>GSHMSMYNMDLDKVIRKINKKGARTVGLQFPEGLKMQAVKIAKAIESQTPATVIISGDPCFGACDVSDYKMKGSVDLIVHYGHTPLPLKYEVPTLFIEAFSNIDVKKDLEKCLEKLEDYSKIALVTTTQHLHLLNEIKDYLEDNGKEVVLGSSKNTKKGQVLGCNFSSIKNLDAEVYLFIGSGNFHPLGIYLFTKSPVLALDPYNSEIRDISAFADRILRIRFARITKAREAEKWGIIVSSKEGQYRMKLAKEIKKILEDNKMEAYIIMADNINPDILLPYMELDAFVVSACPRIAIDDSQMYKKPLLTPQELEIVLNKRQWENYQLDEILFHERYK[2x];>GSGMSRREKMIAKIKDLMYKPDSIRNIGICAHIDHGKTTLSDNLLAGAGMISEELAGDQRFLDFDEQEQARGITIDAANVSMVHNYKDEEYLINLIDTPGHVDFGGDVTRAMRAVDGAVVVVCAVEGIMPQTETVLRQALKENVKPVLFINKVD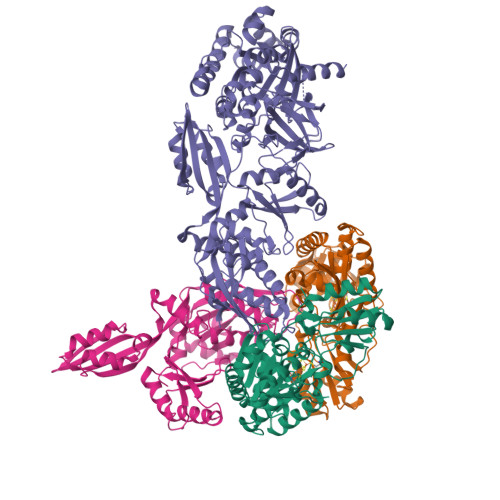RLINELKLEPEELQKRFINIYMEANKLIKNMAPEDKKEEWAVDFTDGSVAFGSAYHNWAINVPMMQETGVNFKDIIDYCNDDKQKELAQKVPLSEVLLGMVVEHLPSPKVSQEYRVPNIWEGDIESPAGQGMITTSPDGPLAVMVTNVSVDKHAGEIATGRVYGGSIEKGTEVYLVGSHSKSRVQQVGVYFGPERVNTDAVPAGNIVYVAGAKGAIAGETICSPEDKIKEFEGLDHISEPVVTVAVEAKNTKDLPKLIEVLRQVAKEDPTIKVEINEETGEHLVSGMGELHLEVISYRIKDKGVEIQTSEPIVVYRETVSQLSPQVEGKSPNKHNRFYITVEPLEDELFKALQEGKLKEGKVKGKESANDFMEYGLDKEEARKVWDVYNRSVFINATRGIQYLDEVKELLIEGFESALNDGPLAKEIAMGLKFKLHDAKLHEDAVHRGPAQVLPAIRNAIYASMMSAGPTLLEPMQKVFINTPQDYMGPCTREIQNRRGQIVDMGQEGDMATIESKVPVAEMFGFAGDIRSAAEGRCLWSTEMSGFERLPREMQNQIVKEIRQRKGLSPEPYGPEHYVG[2x]>MVVKRTMTKKFLEEAFAGESMAHMRYLIFAEKAEQEGFP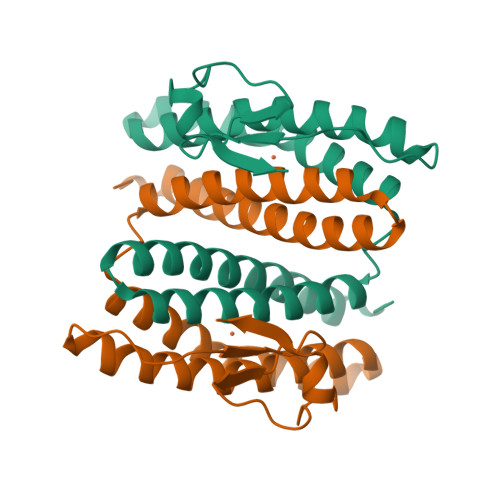NIAKLFRAIAYAEFVHAKNHFIALGKLGKTPENLQMGIEGETFEVEEMYPVYNKAAEFQGEKEAVRTTHYALEAEKIHAELYRKAKEKAEKGEDIEIKKVYICPICGYTAVDEAPEYCPVCGAPKEKFVVFE[2x]>MAMIKMSPEEIRAKSQSYGQGSDQI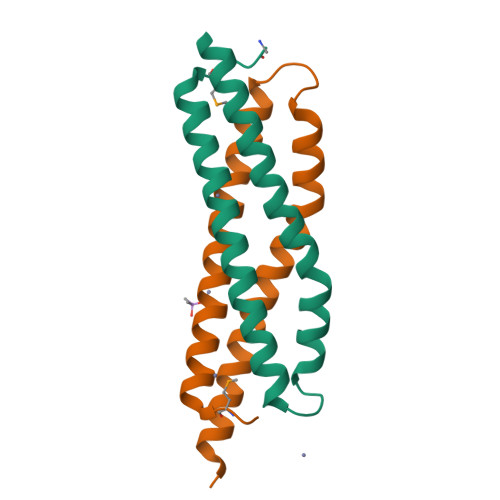RQILSDLTRAQGEIAANWEGQAFSRFEEQFQQLSPKVEKFAQLLEEIKQQLNSTADAVQEQDQQLSNNFGLQ[2x]> MSLHASAIESIETIIVDLPTIRPHKLAMHTMQNQTLVLIRLRCADGIEGLGESTTIGGLAYGNESPDSIKTNIDRFVAPLLIGQDASNINAAMLRLEQSIRGNTFAKSGIESALLDAQGKRLGLPVSELLGGRVRDALPVAWTLASGDTAKDIAEAQKMLDLRRHRIFKLKIGAGEVDRDLAHVIAIKKALGDSASVRVDVNQAWDEAVALRACRILGGNGIDL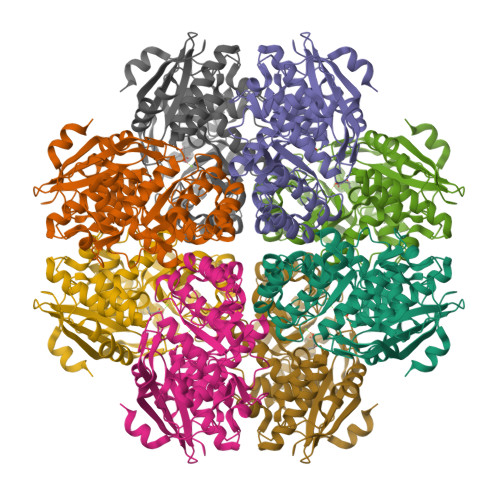IEQPISRNNRAGMVRLNASSPAPIMADESIECVEDAFNLAREGAASVFALKIAKNGGPRATLRTAAIAEAAGIGLYGGTMLEGGIGTLASAHAFLTLNKLSWDTELFGPLLLTEDILAEPPVYRDFHLHVSKAPGLGLSLDEERLAFFRREGHHHHHH Myophage Mu is a representative of contractile nanomachines with a simple tail baseplate. It has the capacity to infect a range of intestinal bacteria and has extensive applications in genetic engineering research. Using cryo-EM, we resolved the three-dimensional (3D) structures of the G(+) type phage Mu in both its extended state and urea-induced contracted state, the latter lacking the baseplate, at near-atomic resolutions. The structure of extended Mu can be divided into four distinct regions: the DNA-containing head, the connector complex, the tail, and the baseplate.

Using icosahedral reconstruction method, a 4.2 Å resolution map of the extended Mu head was generated. The local reconstruction method was employed to improve the resolution of the 3-fold capsid of the head to 3.2 Å. The Mu head is constituted by 415 copies of the MCP gp34, which are organized into 11 pentons and 60 hexons, thereby forming an icosahedral shell with a triangulation number of seven. The MCP gp34 adopts a canonical HK97-like fold. According to the domain nomenclature of MCP gp5 of HK97, each gp34 can be divided into four domains: N-arm, E-loop, P-domain, and A-domain. An asymmetric unit of the icosahedral head comprises seven gp34 monomers (one hexon and one-fifth of a penton). The superimposition of the seven gp34 monomers in an asymmetric unit revealed considerable conformational changes in the N-arms and E-loops, which ultimately led to the formation of capsomers, hexons, and pentons that are assembled into the icosahedral capsid. Despite the absence of cement proteins at inter-capsomere interfaces, complex and extensive interactions are observed around the 3-fold and the quasi-3-fold axes, including hydrogen bonds, salt bridges, and electrostatic interactions. Analogous interactions that reinforce the inter-capsomere stability within the head, independent of cement proteins, have been identified in A-1(L), T7 (47), and R4C.

>[7x]MIVTPASIKALMTSWRKDFQGGLEDAPSQYNKIAMVVNSSTRSNTYGWLGKFPTLKEWVGKRTIQQMEAHGYSIANKTFEGTVGISRDDFEDDNLGIYAPIFQEMGRSAAVQPDELIFKLLKDGFTQPCYDGQNFFDKEHPVYPNVDGTGSAVNTSNIVEQDSFSGLPFYLLDCSRAVKPLIFQERRKPELVARTRIDDDHVFMDNEFLFGASTRRAAGYGFWQMAVAVKGDLTLDNLWKGWQLMRSFEGDGGKKLGLKPTHIVVPVGLEKAAEQLLNRELFADGNTTVSNEMKGKLQLVVADYL> YPGGSTPVS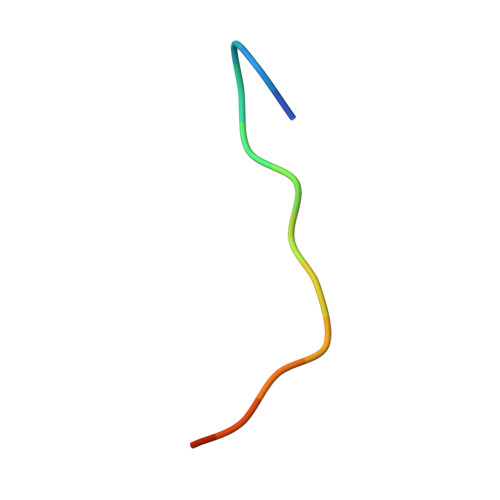SANMM> MSLNITGIQSDWKVEKIEFAKLTGERARSAGANGRIGVHGKSCTVDIARITIDGQTGYGSSIHMTPEWAEDVIGRRLLDLFDDRGRLREAYRLQLEYPVLDWLGQRQGKPVYDLVSGAHLETGASLVVPCYDTSLYFDDLHLADERAAVALMQEEAMQGYAKGQRHFKIKVGRGGRHMPLWEGTKRDIAIVRGISEVAGPAGKIMIDANNAYNLNLTKEVLAALSDVNLYWLEAAFHEDEALYEDLKEWLGQRGQNVLIADGEGLASPHLIEWATRGRVDVLQYDIIWPGFTHWMELGEKLDAHGLRSAPHCYGNAYGIYASGHLSAAVRNFEFVEYDDITIEGMDVSGYRI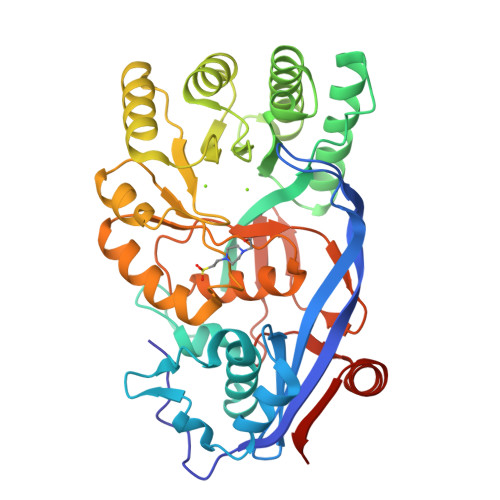ENGEIHVPATPGFGIVFDDELVTYLINRSGWSEGHHHHHH> 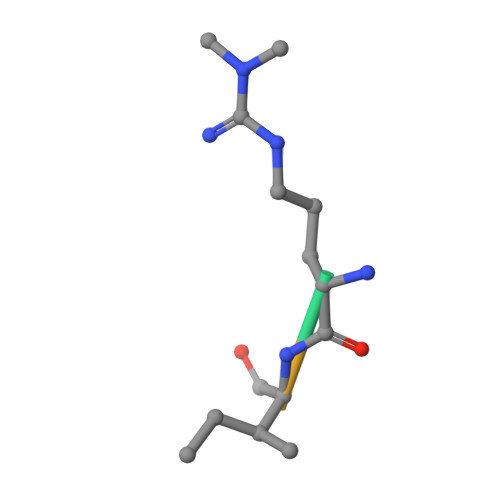RIFS> LWMHKVPASLMVSLGEDAHFQCPHNSSNNANVTWWRVLHGNYTWPPEFLGPGEDPNGTLIIQNVNKSHGGIYVCRVQEGNESYQQSCGTYLRVRQPPPRPFLDMGEGTKNRIITAEGIILLFCAVVPGTLLLFRKRW;> IAELPPKVSVFVPPRDGFFGNPRKSKLICQATGFSPRQIQVSWLREGKQVGSGVTTDQVQAEAKESGPTTYKVTSTLTIKESDWLGQSMFTCRVDHRGLTFQQNASSMCVPDQDTAIRVFAIPPSFASIFLTKSTKLTCLVTDLTTYDSVTISWTRQNGEAVKTHTNISESHPNATFSAVGEASICEDDWNSGERFTCTVTHTDLPSPLKQTISRPKGVALHRPDVYLLPPAREQLNLRESATITCLVTGFSPADVFVQWMQRGQPLSPEKYVTSAPMPEPQAPGRYFAHSILTVSEEEWNTGETYTCVVAHEALPNRVTERTVDKSTEGEVSADEEGFENLWATASTFIVLFLLSLFYSTTVTLF;> SRIWQSPRFIARKRGFTVKMHCYMNSASGNVSWLWKQEMDENPQQLKLEKGRMEESQNESLATLTIQGIRFEDNGIYFCQQKCNNTSEVYQGCGTELRVMGFSTLAQLKQRNTLKDGIIMIQTLLIILFIIVPIFLLLD;> IAELPPKVSVFVPPRDGFFGNPRKSKLICQATGFSPRQIQVSWLREGKQVGSGVTTDQVQAEAKESGPTTYKVTSTLTIKESDWLGQSMFTCRVDHRGLTFQQNASSMCVPDQDTAIRVFAIPPSFASIFLTKSTKLTCLVTDLTTYDSVTISWTRQNGEAVKTHTNISESHPNATFSAVGEASICEDDWNSGERFTCTVTHTDLPSPLK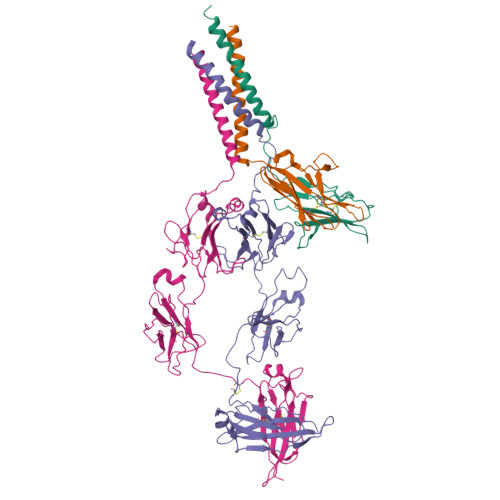QTISRPKGVALHRPDVYLLPPAREQLNLRESATITCLVTGFSPADVFVQWMQRGQPLSPEKYVTSAPMPEPQAPGRYFAHSILTVSEEEWNTGETYTCVVAHEALPNRVTERTVDKSTEGEVSADEEGFENLWATASTFIVLFLLSLFYSTTVTLFK Rab proteins, the biggest subfamily within the superfamily of small GTPases, are major regulators of vesicular trafficking in eukaryotic cells. One such family of effector proteins that was reported to link Rab proteins and the cytoskeleton is the Mical (molecules interacting with CasL) family. In this publication, we present a thorough biochemical and structural analysis of a Rab effector domain termed bivalent Mical/EHBP Rab binding (bMERB) domain. The results show that the domains probably constitute a Rab8-effector family involved in endosomal trafficking, and the Rab-binding specificity can be well explained from the 3-dimensional structures of complexes determined in this work.

Stimulated by the evidence for two Rab binding sites in some bMERB domains (Mical-1, Mical-3 and EHBP1L1), we searched for crystallization conditions of these RBDs with Rabs in a 1:2 stoichiometry. Crystallization conditions were found using a complex of Rab101–175 and the RBD of Mical-1 (residues 918–1067), yielding crystals that diffracted to a resolution of 2.8 Angstrom at a synchrotron X-ray source and the resulting structure indeed showed two molecules of Rab10 bound to Mical-1. Whereas one Rab protein binds to α-helix 1 and the first half of α-helix 2 (Mical-1918-991, binding site 1, blue), the second molecule of Rab10 binds the second half of α-helix 2 and α-helix 3 (Mical-1994-1060, binding site 2, green). Upon superimposition of both binding sites, the strong similarity becomes obvious and the helices from both binding sites adopt very similar positions. Upon closer inspection and alignment, a strong similarity between the two Rab binding sites in Mical-1 became obvious, involving the same/similar residues both within the two different molecules of Rab10 as well as the two binding sites in Mical-1, respectively. Consistent with the localization of the two separate binding sites within the N-terminal and the C-terminal half of the bMERB domain, respectively, deletion constructs lacking either α-helix 1 (Mical960–1067) or α-helix 3 (Mical-1918–1020) displayed a clear 1:1 stoichiometry of Rab binding both in aSEC and ITC experiments. Furthermore, the ITC data allowed us to clearly allocate the high affinity binding to the C-terminal binding site and the lower affinity binding to the N-terminal binding site. In summary, the strong conservation of interacting residues between both sites as well as the structural conservation of the binding sites lead us to conclude that this family of Rab binding proteins must have evolved via gene duplication. The work presented constitutes the first description of two Rab proteins binding a single effector domain.

>[2x]GHMAKKTYDLLFKLLLIGDSGVGKTCVLFRFSDDAFNTTFISTIGIDFKIKTVELQGKKIKLQIWDTAGQERFHTITTSYYRGAMGIMLVYDITNGKSFENISKWLRNIDEHANEDVERMLLGNKCDMDDKRVVPKGKGEQIAREHGIRFFETSAKANINIEKAFLTLAEDILRKTP;> GHMKEEEMKRFCKAQTIQRRLNEIEAALRELEAEGVKLELALRRQSSSPEQQKKLWVGQLLQLVDKKNSLVAEEAELMITVQELNLEEKQWQLDQELRGYMNREENLKTAADRQAEDQVLRKLVDLVNQRDALIRFQEERRLSELALGTGAQG> ASVHGTTYELLRRQGIDTVFGNPGSNELPFLKDFPEDFRYILALQEACVVGIADGYAQASRKPAFINLHSAAGTGNAMGALSNAWNSHSPLIVTAGQQTRAMIGVEALLT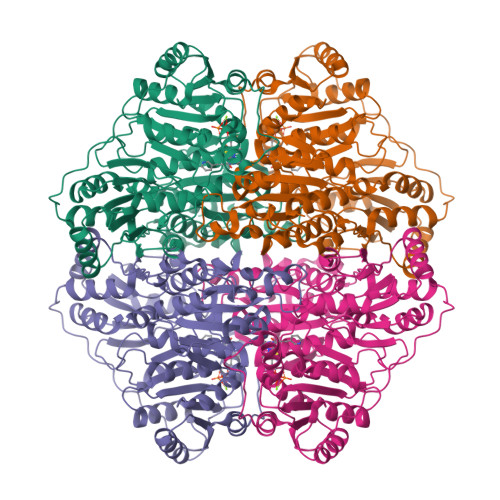NVDAANLPRPLVKWSYEPASAAEVPHAMSRAIHMASMAPQGPVYLSVPYDDWDKDADPQSHHLFDRHVSSSVRLNDQDLDILVKALNSASNPAIVLGPDVDAANANADCVMLAERLKAPVWVAPSAPRCPFPTRHPCFRGLMPAGIAAISQLLEGHDVVLVIGAPVFRYHQYDPGQYLKPGTRLISVTCDPLEAARAPMGDAIVADIGAMASALANLVEESSRQLPTAAPEPAKVDQDAGRLHPETVFDTLNDMAPENAIYLNESTSTTAQMWQRLNMRNPGSYYFCAAGGLGFALPAAIGVQLAEPERQVIAVIGDGSANYSISALWTAAQYNIPTIFVIMNNGTYGALRWFAGVLEAENVPGLDVPGIDFRALAKGYGVQALKADNLEQLKGSLQEALSAKGPVLIEVSTVSP>MIVAEIQKNSLKEQRIKFIRNHQQAFDVEPIYPLRLFEDFVMSVEGDCSIEASCKIELDKLIASRFMLFFKDQEWEKYLTQSLAFFRQVENRVGVQLDYSLLQKFLGHNFDFSKLEVLSAGLDLRTNLADSSLKIHIRIKDYPEKINQALSLTIDGDDLTAVRDFLSVVGFDFYFDGRSAIEIYPEVKKEDFFKPKTQEKVWQHLPKFVLEPLQVTNLFGFGFSKTNHNPVVYYRLKGRQDLTNYFKINDTAQRVHSFYQHQDILPNMWVGTTQKELE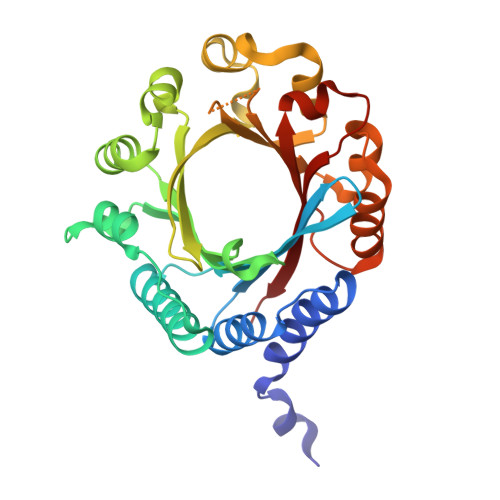KTRIENIRLYYYKSFKM[2x]> MKKQNDIPQPIRGDKGATVKIPRNIERDRQNPDMLVPPETDHGTVSNMKFSFSDTHNRLEKGGYAREVTVRELPISENLASVNMRLKPGAIRELHWHKEAEWAYMIYGSARVTIVDEKGRSFIDDVGEGDLWYFPSGLPHSIQALEEGAEFLLVFDDGSFSSTFQLTDWLAHTPKEVIAANFGVTKEEISNLPGKEKYIFENQLPGSLKDDIVEGPNGEVPYPFTYRLLEQEPIESEGGKVYIADST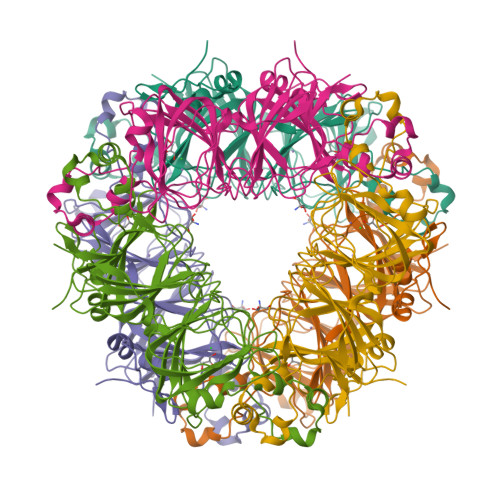NFKVSKTIASALVTVEPGAMRELHWHPNTHEWQYYISGKARMTVFASDGHARTFNYQAGDVGYVPFAMGHYVENIGDEPLVFLEIFKDDHYADVSLNQWLAMLPETFVQAHLDLGKDFTDVLSKEKHPVVKKKCSK>[2x]EKQPNIDELKKRMEQSRPNKLRGDLDQLIESDPKLRALRPHLKIDLVQEGLRIQIIDSQNRPMFKTGSAEVEPYMRDILR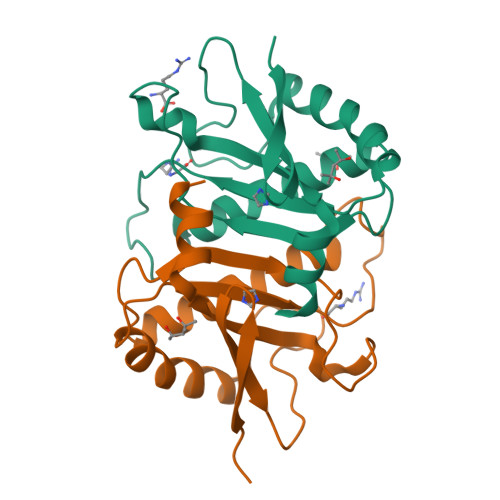AIAPVLNGIPNRISLAGHTDDFPYANGEKGYSNWELSADRANASRRELVAGGLDNGKVLRVVGMAATMRLSDRGPDDAINRRISLLVLNKQAEQAILHHHHHH>[3x]MEIDKELAPQDRTVTVATVLPTVPGPSPFTIKQPFQSEVL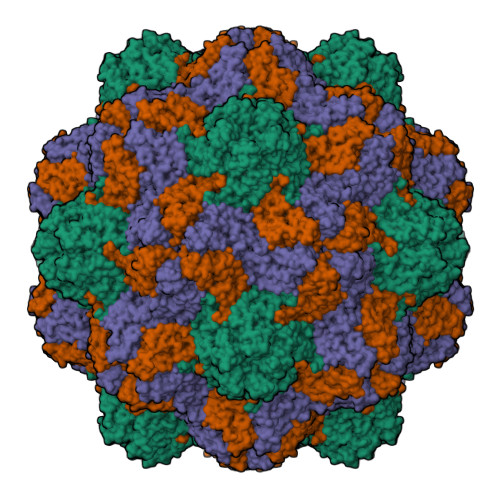FAGTKDAEASLTIANIDSVSTLTTFYRHASLESLWVTIHPTLQAPAFPTTVGVCWVPAQSPVTPTQITKTYGGQIFCIGGAIQTLSPLIVKCPLEMMQPRVKDSIQYLDSPKLLISITAQPTAPPASTCIITVSGTLSMHSPLITDTST> MKLLHERMMHSLARYPRQTAVVDEQDALSYEALELRIREFVAMLCALGVGQGQRILLWAHKSVDLVAVMQAALRLGVVYVPVDPLSPVSRLEKIAGDSQAVLVLCTAARLEELAGSALAQVRSVVLDDPASAGYWRNIDTGSSVVPTLAIQPDDLAYILYTSGSTGVPKGVALSHGNALAFVDWACERYCFQPGERFANHAPLHFDLSVLDIYCALNVGATVCLVPESIAFSPRLLTDFIRQHEISI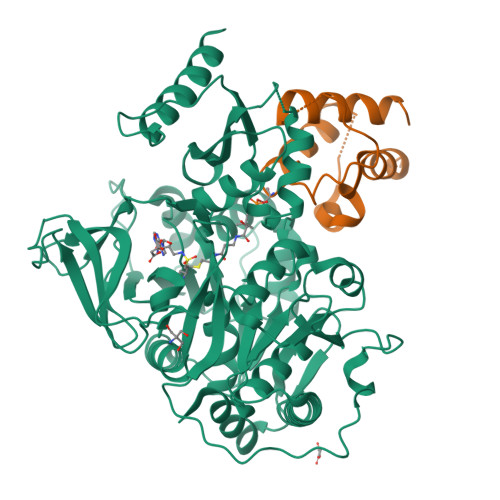WYSVPSVLMMMMQDGDLLSDIQDTLRVLLFAGEPFPVKHLRDLRAAYADVRLANLFGPTETNVCTAFEVGAIDPERVLPVPIGTAASGNQVWAQKPDGSRCAVGEEGELVVQGPTVMLGYFAKPAQEGPYKTGDMVRQRPDGNYEYLGRRDDMLKVRGNRIERGEVEAALLAHPQVSEAAVLVVGEGMNAQLWGVLVAHTRDALSLIDLKRHCAQRLPRYMIIDKVLCLDALPRNANGKVDRFALARQVEGKLAAALEHHHHHHHH;> MDGEEVKEKIRRYIMEDLIGPSAKEDELDDQTPLLEWGILNSMNIVKLMVYIRDEMGVSIPSTHITGKYFKDLNAISRTVEQLKAESALEHHHHHH4-(2-methylpropyl)benzoic 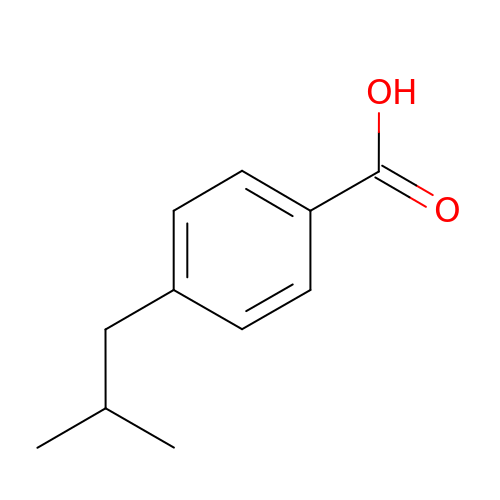acid | C11 H14 O2 | VUBBCFWWSKOHTH-UHFFFAOYSA-N>[2x]AFYKREMFDPAEKYKMDHRRRGIALIFNHERFFWHLTLPERRGTCADRDNLTRRFSDLGFEVKCFNDLKAEELLLKIHEVSTVSHADADCFVCVFLSHGEGNHIYAYDAKIEIQTLTGLFKGDKCHSLVGKPKIFIIQACRGNQHDVPVIPLDVVDAASVYTLPAGADFLMCYSVAEGYYSHRETVNGSWYIQDLCEMLGKYGSSLEFTELLTLVNRKVSQRRVDFCKDPSAIGKKQVPCFASMLTKKLHFFPKSNGNSHHHHHH

Caspases are a family of cysteinyl proteases that are key mediators of apoptosis and inflammation. The apoptotic “executioner” caspases (caspases-3, -6 and -7) are translated as proenzymes containing a short pro-domain, a p20 subunit, a linker region, and p10 subunit. The resulting active enzyme is a dimer, wherein each subunit contains a p10 and p20 chain and one active site. Due to the role of caspase-6 in neurodegeneration, there is strong interest in developing selective, small-molecule inhibitors of this enzyme.

We first generated a binary complex of caspase-6 with a substrate surrogate covalently bound to the catalytic cysteine (Cys163) by incubating active caspase-6 with a covalent inhibitor (benzyloxycarbonyl (Z)-VEID-tetrafluorophenoxymethyl ketone). The unambiguous electron density for 3 reveals a unique simultaneous binding of substrate and inhibitor that explains the uncompetitive behavior of this series. The carbonyl group of 3 makes a 3.1-Å hydrogen bond with the backbone NH of the P2 Ile of the bound VEID substrate surrogate. The dimethoxyphenyl ring of 3 sits above the oxyanion hole created by the backbone NH group of Cys163; the 4-methoxy phenyl group displaces the water network around the His121-Cys163 catalytic dyad and the scissile bond. The primary alcohol of 3 makes a hydrogen bond interaction with the P3 Glu of VEID and participates in a water-mediated interaction with Arg220 of the L3 loop of caspase-6. The benzonitrile ring of 3 overlaps with the S4 subsite and tucks under the L4 loop of caspase-6, which places the nitrile group close to the sidechains of His168 from the L2 loop and His219 from the L3 loop. The slight difference in the conformation of the L4 loop in the ternary complex in comparison to the conformation in the binary complex is likely due to the benzonitrile ring interaction with residues at the tip of the L4 loop. To better understand this selectivity profile, we superposed the caspase-3/DEVD coordinates onto the caspase-6/VEID/3 ternary structure. Three residues lining the binding site of 3 provide a structural rationale for the selectivity of these inhibitors (Cys264 and Ala269 in the L4 loop and His209 in the L3 loop); we believe that Ala269 is the primary driver of caspase selectivity (amino acids depicted in Figure 5C). The x-ray structure lacks the Rh110 dye, indicating that compound 3 can bind to the VEID/caspase-6 complex in the absence of a prime-side dye.>MVYQVKDQEDFTKQLNEAGNKLVVIDFYATWCGPCKMIAPKLEELSQSMSDVVFLKVDVDECEDIAQDNQIACMPTFLFMKNGQKLDSLSGANYDKLLELV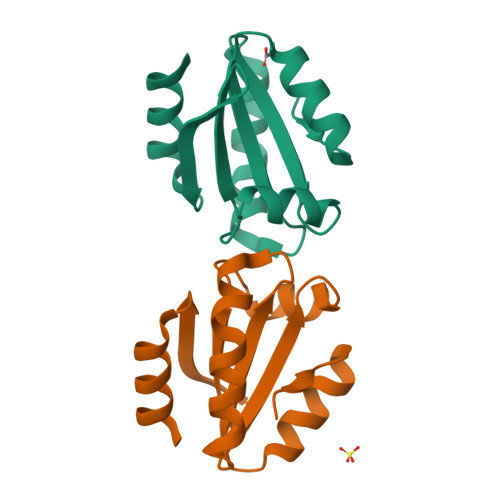EKNK[2x]>GLPNNICLQKTSNQILKPKLISYTLPVVGQSGTCITDPLLAMDEGYFAYSHLERIGSCSRGVSKQRIIGVGEVLDRGDEVPSLFMTNVWTPPNPNTVYHCSAVYNNEFYYVLCAVSTVGDPILNSTYWSGSLMMTRLAVKPKSNGGGYNQHQLALRSIEKGRYDKVMPYGPSGIKQGDTLYFPAVGFLVRTEFKYNDSNCPITKCQYSKPENCRLSMGIRPNSHYILRSGLLKYNLSDGENPKVVFIEISDQRLSIGSPSKIYDSLGQPV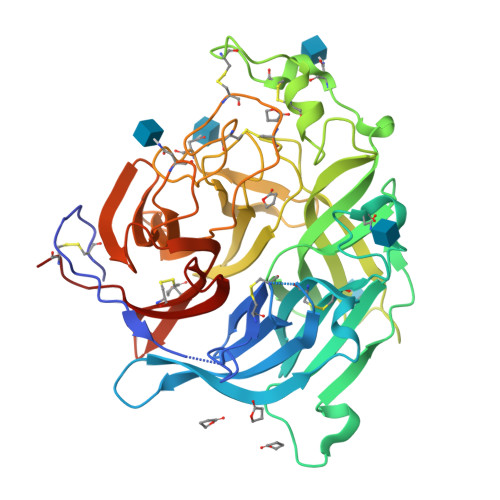FYQASFSWDTMIKFGDVLTVNPLVVNWRNNTVISRPGQSQCPRFNTCPEICWEGVYNDAFLIDRINWISAGVFLDSNQTAENPVFTVFKDNEILYRAQLASEDTNAQKTITNCFLLKNKIWCISLVEIYDTGDNVIRPKLFAVKIPEQCT[2x]> MTPKTETPVGALIKKFFPGKRFQKNYLKDAGKKLKREGEAAAVEYLSGKQEDHPANFCPPAKVNILAQSRPLSEWPINLVSKGVQEYVYGLTAAEREANGDFGTSRKSLDRWFARTGVPTHGYTTVQGLNLILRHTFNRYDGVIKKVETRNEKRRSKATRINVSREADGLPPIEAEPEETAFGPDGKLKERPGINPSIYCYQQVSPVPYNPAKHPALPFSGVDPGAPLPLGTPNRLSIPKGQPGYVPEWQRPHLSTKNKRIRKWYARANWRRKPGRKSVLDEAKLKEAALKEAIPIIVTIGKDWIVMDARGLLRAVYWRGIAKPGLSLKELLGFFSGDPVLDPKRGIATFTFKLGAVAVHSRKPTRGKKSKELLLSMTAEKPHVGLVAIDLGQTNPVAAEFSRVKREGETLQAEPLGQIVLPDDLVKDLTRYRRAWDATEEQIKAEAIVQLPEECRAEVVKVNQMSAEETKHLILDRGVSGDLPWEKMTSNTTFISDHLLAKGVTDQVFFEKKSKGKKKGTETVKRKDYGWVKLLRPRLSQETRKAVNDKTWELKRASTEYVRLSRRKTELARRCVNYIVRETKRWTQCEDIAIVIEDLNVRFFHGSGERPDGWDNFFISKRENRWFIQ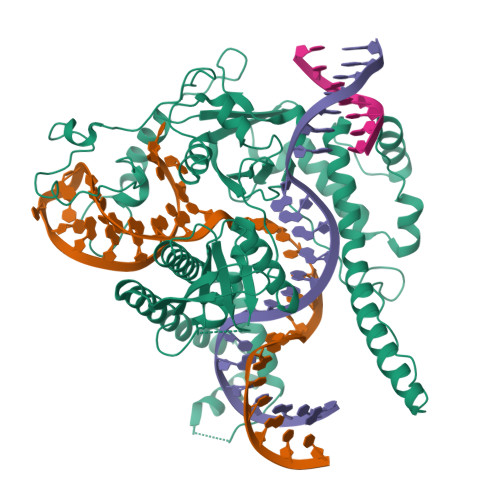VLHKAFSDLALHRGLPVIEANPARTSITCIRCGHCDRNNRHGEMFLCLSCNDLRHADREIATRNLTRVAVTGEMIPRRIEPGEQSGDTKKARSARKGKKAVISKREAA>[2x]MTDILIDDTATEAVRTLIRAFPLVPVSQPPEQGSYLLAEHDTVSLRLVGEKSNVIVDFTSGAAQYRRTKGGGELIAKAVNHTAHPTVWDATAGLGRDSFVLASLGLTVTAFEQHPAVACLLSDGIRRALLNPETQDTAARINLHFGNAAEQMPALVKTQGKP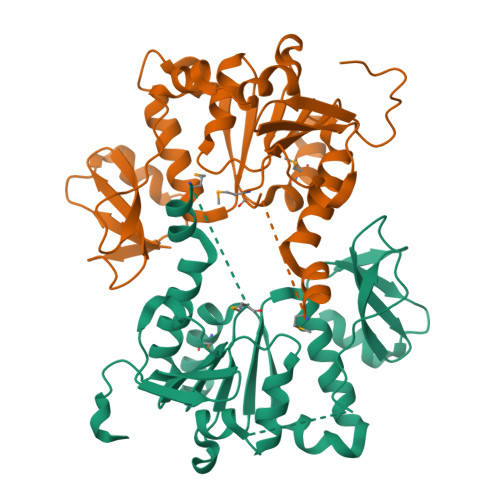DIVYLDPMYPERRKSAAVKKEMAYFHRLVGEAQDEVVLLHTARQTAKKRVVVKRPRLGEHLAGQAPAYQYTGKSTRFDVYLPYGADKGLEHHHHHH> GHMTIARDIVLQESVGKGRFGEVWRGKWRGEEVAVKIFSSREERSWFREAEIFQTVMLRHENILGFIAADNKDNGTWTQLWLVTDFHEHGNLFDYLNRYTVTVEGMIKLALSTASGLAHLHMEIVGTQGKPAIAHRDLKSKNILVKKNGTCCICDFGLAVRHDSATDTID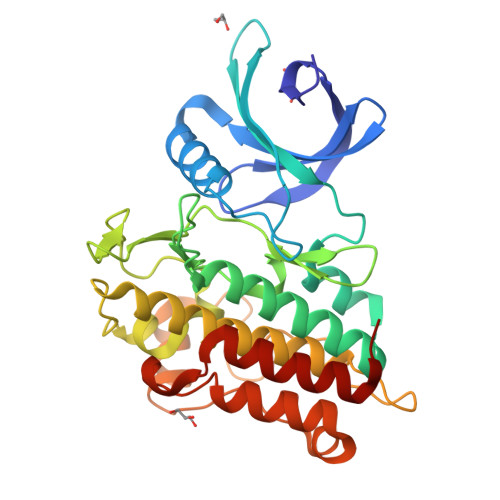IAPNHRVGTKRYMAPEVLDDSINMKHFESFKRADIYAMGLVFWEIARRCSIGGIHEDYQLPYYDLVPSDPSVEEMRKVVCEQKLRPNIPNRWQSCEALRVMAKIMRECWYANGAARLTALRIKKTLSQLSQQEGIKM> MRLLYLHADRFEYKTVKPALKNPPDPPGEASFGEALVVFTTVEDGDGPQTVMYAASDIASHSSRLKVTTVILY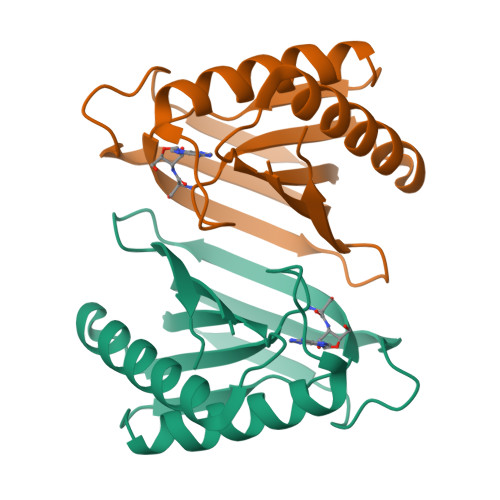PYAHLSSRLAKPMAAHKRLIELEGALRTKFPGHVHRAPFGWYKSFSIACKGHPLAALSRSFTE> MEKTEKNELVRKLIFNPQGDREASKRKIIKGNPTNIFELNEIKYSWAFDLYKLMGFTNFWIPEEIQMLEDRKQYETVLSDYEKRAYELVLSFLIALDSFQVDMLKEFGRMITAPEVEMAITAQEFQESVHAYSYQFILESVVDPVKADEIYNYWRE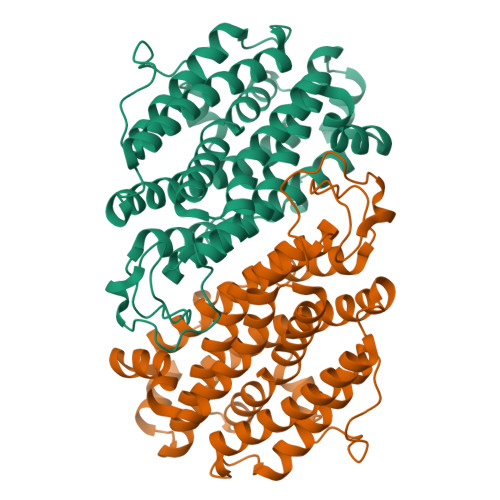DERLLERNKVIAELYNEFIRKPNEENFIKATIGNYILESLYFYSGFAFFYTLGRQGKMRNTVQQIKYINRDELCHVTLFRNIINTLRKENPELFTPEIEKWIVEYFKYAVNEEIKWGQYVTQNQILGINDVLIERYIKYLGNLRITQIGFDPIYPEVTENPLKWIDEFRKINNTKTDFFQAKPQTYSKANELKW> HHHHHHTDPALRAAQQTPLYEQHTLCGARMVDFHGWMMPLHYGSQIDEHHAVRTDA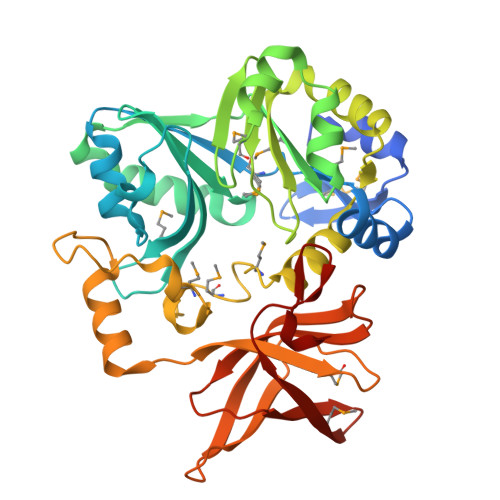GMFDVSHMTIVDLRGSRTREFLRYLLANDVAKLTKSGKALYSGMLNASGGVIDDLIVYYFTEDFFRLVVNSATREKDLSWITQHAEPFGIEITVRDDLSMIAVQGPNAQAKAATLFNDAQRQAVEGMKPFFGVQAGDLFIATTGYTGEAGYEIALPNEKAADFWRALVEAGVKPCGLGARDTLRLEAGMNLYGQEMDETISPLAANMGWTIAWEPADRDFIGREALEVQREHGTEKLVGLVMTEKGVLRNELPVRFTDAQGNQHEGIITSGTFSPTLGYSIALARVPEGIGETAIVQIRNREMPVKVTKPVFVRNGKAVAGLCGR>GMELQDTIFKRQSVRKFKNQDVSDEDILKMIKAAGAAPSGKNIQNWHFVVIKRRDLMEKIADVITKKQQEILVEMDKVSVDKANRFRKFVKNFTLFYLKAPVLVLVFTKVYNPSGYYELELIDAPKETIDKLFIRNPGMQ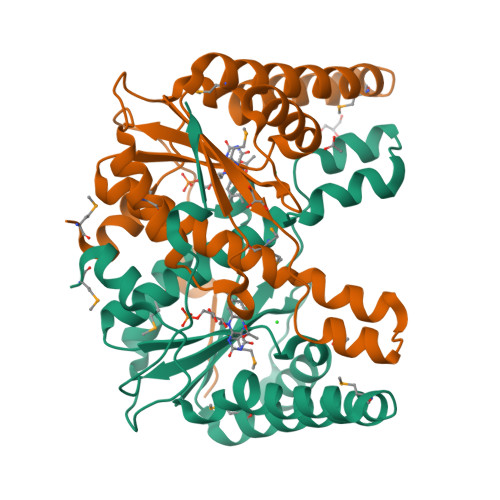SLGAAIENFTLSAIELGYGSCWLTSQNYAADEIEAVLEAETGFEKGEYFLGAMLALGVPEDNLKSPSKKPVEEICTFIK[6x]Neurexins are presynaptic, cell‐adhesion molecules that specify the functional properties of synapses via interactions with trans‐synaptic ligands. Neurexophilins are a family of secreted, neuropeptide‐like glycoproteins originally discovered as α‐neurexin ligands and later found to bind to the LNS2 domain of α‐neurexins (Petrenko et al, 1996; Missler et al, 1998; in the following we often refer to α‐neurexins simply as neurexins or Nrxns). Here, we determined high‐resolution structures of the complex of neurexophilin‐1 and the second laminin/neurexin/sex‐hormone‐binding globulin domain (LNS2) of neurexin‐1 and examined how alternative splicing at splice site #2 (SS2) regulates the complex. Our data reveal a unique, extensive, neurexophilin–neurexin binding interface that extends the jelly‐roll β‐sandwich of LNS2 of neurexin‐1 into neurexophilin‐1.

In the structure of the Nxph1‐LNS2SS2A+ complex, the 384‐HAM‐386 sequence of SS2A extends the N‐terminal part of LNS2 β9. The other part of the SS2A sequence (379‐HSGIG‐383) forms a disordered, solvent‐exposed loop as suggested by corresponding weak electron density. Difference density maps calculated by subtracting the observed structure factor amplitudes of the Nxph1‐LNS2SS2− structure from those of the Nxph1‐LNS2SS2A+ structure showed strong positive electron density throughout the region near SS2A. Strong positive difference peaks revealed the extension of the β9 384‐HAM‐386 part of the SS2A insert sequence in the Nxph1‐LNS2SS2A+ structure. Furthermore, the M386 and H384 residues of SS2A extend across β10 of LNS2 to interact with H125 on β1 of Nxph1. Specifically, in the Nxph1‐LNS2SS2A+ structure, but not the Nxph1‐LNS2SS2− structure, L376 points into the core of the molecule toward L346, which shifts along with the backbone of β7 further into the core of the molecule. In addition, there is a shift of Y407 into the core of the LNS2 molecule in the Nxph1‐LNS2SS2A+ structure. Taken together, these structures show that SS2A adds specific inter‐molecular interactions to the Nxph1‐LNS2 interface while also inducing regional conformational changes to stabilize the complex. Indeed, Nxph1 binds to Nrxn1 LNS2SS2A+ with ~6‐fold higher affinity than for Nrxn1 LNS2SS2−. For example, the Nxph1‐LNS2SS2A+ interface contains the same key I401 residue found interdigitating with Nxph1 at the Nxph1‐LNS2SS2− interface.

> DASIATFKGSEYFCYDLSQNPIQSSSDEITLSFKTLQRNGLMLHTGKSADYVNLALKNGAVSLVINLGSGAFEALVEPVNGKFNDNAWHDVKVTRNLRQHSGIGHAMVTISVDGILTTTGYTQEDYTMLGSDDFFYVGGSPSTADLPGSPVSNNFMGCLKEVVYKNNDVRLELSRLAKQGDPKMKIHGVVAFKCAALEVLFQ;> DAAQPAARDFGWGDFHSNIKTVKLNLLITGKIVDHGDGTFSVYFRHDSTGQGDVSVSLVPPTKIVEFDLAQQTVIDAKDSKSFNCRIEYEKVDKATKNTLCNYDPSKTCYQEQTQSHVSWLCSKPFKVICIYISFYSTDYKLVQKVCPDYNYHSDTPYFPSGLEVLFQ>GGTNDAFSLSFETNNTPRMTIDDVGRVGVGTTAPTSALHVIGTGEVARFVTSATGGVVIDSTALNYNPSLIYRKTNINRWSMMVNAASETGGNAGSNLSILRYDDTGATLGAAVTIDRASGFFGINTAAPAYNIH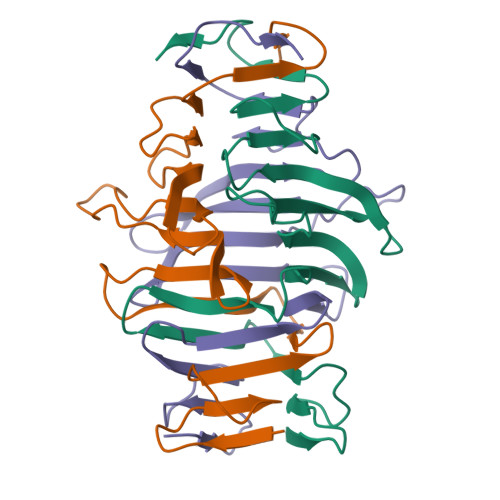VTGTAGLSTGSAWTVAS[6x]>GPLGSPEF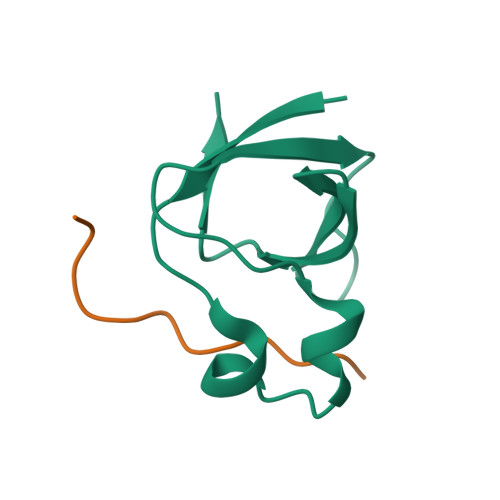RYFVAMFDYDPSTMSPNPDGCDEELPFQEGDTIKVFGDKDADGFYWGELRGRRGYVPHNMVSEVE[10x];>[10x]XIGRRLPPTPSKPSTLX>[2x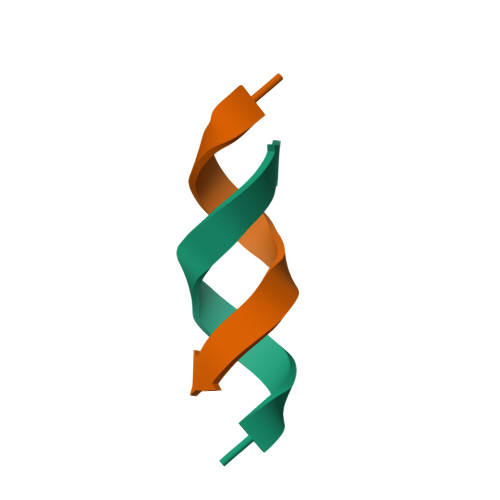]YYYYYYYYK>[2x]MATGLALETKDGLHLFGRNMDIEYSFNQSIIFIPRNFKCVNKSNKKELTTKYAVLGMGTIFDDYPTFADGMNEKGLGCAGLNFPVYVSYSKEDIEGKTNIPVYNFLLW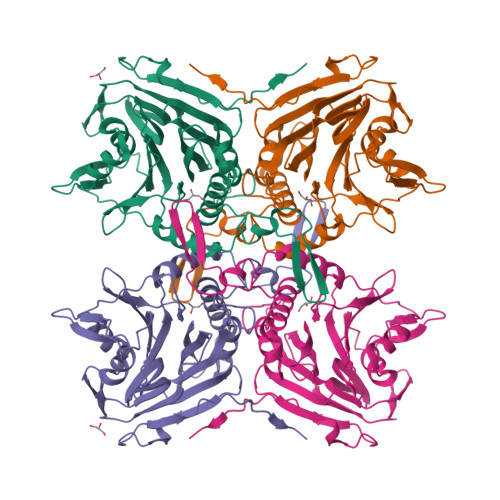VLANFSSVEEVKEALKNANIVDIPISENIPNTTLHWMISDITGKSIVVEQTKEKLNVFDNNIGVLTNSPTFDWHVANLNQYVGLRYNQVPEFKLGDQSLTALGQGTGLVGLPGDFTPASRFIRVAFLRDAMIKNDKDSIDLIEFFHILNNVAMVRGSTRTVEEKSDLTQYTSCMCLEKGIYYYNTYENNQINAIDMNKENLDGNEIKTYKYNKTLSINHVN>ARSEKRVPMTRLRKRVAERLLEAKNSTAMLTTFNEVNMKPIMDLRKQYGEAFEKRHGIRLGFMSFYVKAVVEALKRYPEVNASIDGDDVVYHNYFDVSMAVSTPRGLVTPVLRDVDTLGMADIEKKIKELAVK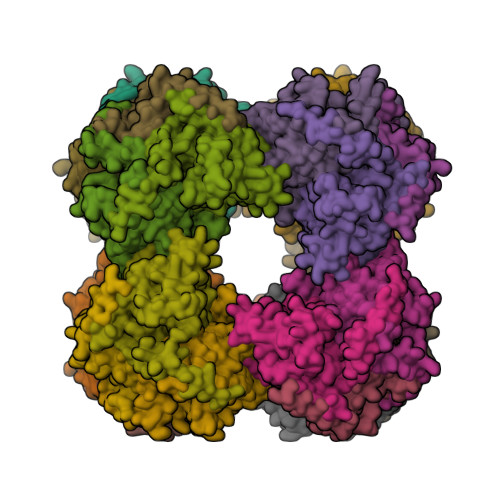GRDGKLTVEDLTGGNFTITNGGVFGSLMSTPIINPPQSAILGMHAIKDRPMAVNGQVEILPMMYLALSYDHRLIDGRESVGFLVTIKELLEDPTRLLLDV[6x]> HHHHHHGSMKKILIALISFAFAVSCKAPQKEEPINITPEELDASIDRVTEIMIHDIFSPPVASRIFAYPNVAAYEIVAATNDNYNSLAGQLNGLTAIPEPDTTKTINYELAAVVAHMELSKRLIFSEDRMESLRDSLYMVWEGKNPVLFSDSKAYGLQVADHIGEWMNKDNYAQTRTMPKFTVDADDPGRWQPTPPAYMDGIEPHWNKIRPFVLDSAAQFKPVPPPAYSLEEDSAFYKELKEVYDVRNKITEEGDSSEEIQIARFWDCNPYVSVTRGHLMFATKKITPGAHWMGIAKIAARKTNSDFAKTLFAYTKASVAMADAFISCWDEKYRSNLIRPETVINQHIDDSWK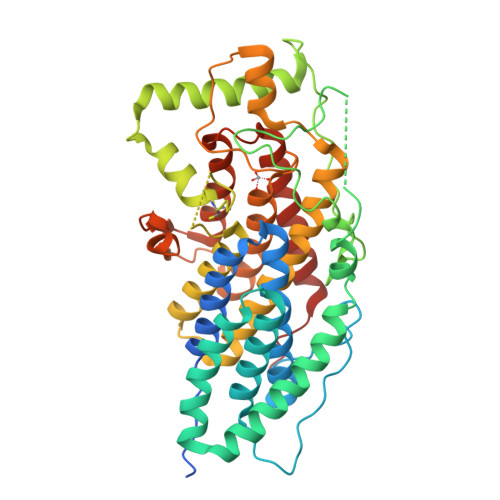PVLQTPPFPEYTSGHSVVSGAASVVLTEVFGDNFSFDDDTEVPYGLPIRSFKSFKQAADEAAISRMYGGIHYRAAIEVGVKQGRDLGTFVVNKLHMLSDKKVAQN>[4x]AQVKKLVIRVHMSDDSSKTMMVDERQTVRQVLD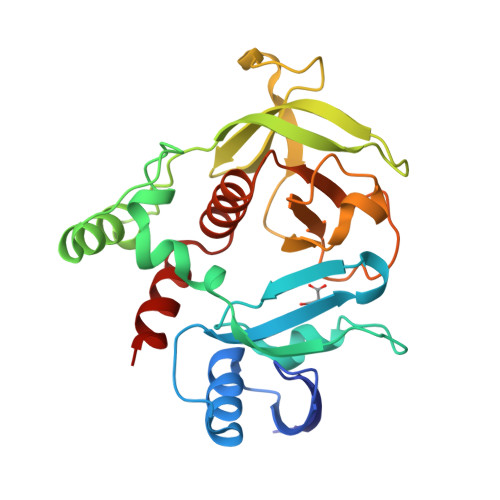NLMDKSHCGYSLDWSLVETVSELQMERIFEDHENLVENLLNWTRDSQNKLIFMERIEKYALFKNPQNYLLGKKETAEMADRNKEVLLEECFCGSSVTVPEIEGVLWLKDDGKKSWKKRYFLLRASGIYYVPKGKAKVSRDLVCFLQLDHVNVYYGQDYRNKYKAPTDYCLVLKHPQIQKKSQYIKYLCCDDVRTLHQWVNGIRIAKYGKQLYMNYQEALKRT> MHHHHHHHHTFTRYSRLRVIAEIRHGDIFHSANIVSSIEFDRDDELFATAGVSRCIKVFDFSSVVNEPADMQCPIVEMSTRSKLSCLSWNKHEKNHIASSDYEGIVTVWDVTTRQSLMEYEEHEKRAWSVDFSRTEPSMLVSGSDDCKVKVWCTRQEASVINIDMKANICCVKYNPGSSNYIAVGSADHHIHYYDLRNISQPLHVFSGHKKAVSYVKFLSNNELASASTDSTLRLWDVKDNLPVRTFRGHTNEKNFVGLTVNSEYLACGSETNEVYVYHKEITRPVTSHRFGSPDMDDAEEEAGSYFISAVCWKSDSPTMLTANSQGTIKVLVLAA;> IESDEEIRRVPE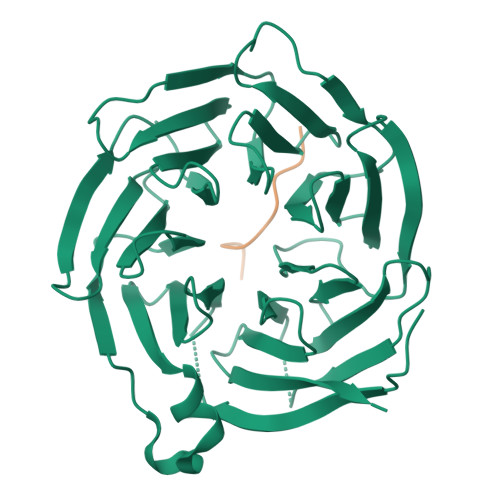FGGEAVG>MAEAEAGGDEARCVRLSAERAKLLLAEVDTLLFNCDGVLWRGETAVPGAPETLRALRARGKRLGFITNNSSKTRTAYAEKLRRLGFGGPVGPEAGLEVFGTAYCSALYLRQRLAGVPDPKAYVLGSPALAAELEAVGVTSVGVGPDVLHGDGPSDWLAVPLEPDVRAVVVGFDPHFSYMKLTKAVRYLQQPDCLLVGTNMDNRLPLENGRFIAGTGCLVRAVEMAAQRQADIIGKPSRFIFDCVSQEYGINPERTVMVGDRLDTDILLGSTCSLKTILTLTGVSSLEDVKSNQESDSMFKKKMVPDFYVDSIADLLPALQG[8x]

Phosphoglycolate phosphatase (PGP, also called glycerol 3-phosphate phosphatase or AUM11) is an evolutionarily conserved metabolite damage control enzyme that can dephosphorylate and thereby repair three adventitious glycolytic metabolites: 2-phospho-L-lactate, 4-phosphoerythronate, and 2-phosphoglycolate. PGP belongs to the haloacid dehalogenase (HAD)-type superfamily of phosphatases, a large, widespread and evolutionarily ancient class of hydrolases with emerging roles in human physiology and disease. All HAD phosphatases consist of a catalytic core domain with a Rossmanoid-fold. This core is accessorized with so-called cap domains, which are mobile elements that can shield the entry to the catalytic cleft.

We had shown earlier that PGP exists in a dynamic equilibrium between homodimers and -tetramers, and that the mutation of Cys297 to Ser (PGPC297S) abolished disulfide-mediated PGP tetramer formation. For subsequent crystallization attempts, we additionally exchanged the catalytically essential Asp34 to Asn, which abolishes PGP activity towards its substrates. Full-length murine PGPD34N/C297S (here referred to as apo-PGP) crystallized in space group P1 with four dimers per asymmetric unit, referred to as AB, CD, EF and GH dimers. While monomers A-F and H are well defined in the electron density maps, large sections of the catalytic core of monomer G display very weak density. An inspection of the PGP catalytic cleft showed that the active site of PGP is organized as a channel, and that Asn34 (corresponding to the Asp34 nucleophile) is centrally buried within this cleft. Coupled to this rotation is a shift of the substrate specificity loop (amino acids 202–215) by up to ~6 Å for corresponding Cα atoms towards the catalytic core. Conversely, the cap domains (Cα atoms of residues 100–237) can be superimposed, which then identifies a movement of the PGP ‘flap’ (amino acids 39–46 of the core domain) by >5 Å towards the catalytic core. Upon rotation of the substrate specificity loop and the flap, channel entrances become obstructed, and access to the active site is blocked. To our knowledge, experimental proof for the existence of open (chains D and E) and closed (chains A-C, F and H) conformations in a C2-capped mammalian phosphatase has not been previously provided.> MKPEVEQELAHILLTELLAYQFASPVRWIETQDVFLKDFNTERVVEIGPSPTLAGMAQRTLKNKYESYDAALSLHREILCYSKDAKEIYYTPDPSELAAKEEPAKEEAPAPTPAANAPAPAAAAPAPVAAAAPAAAAAEIADEPVKASLLLHVLVAHKLKKSLDSIPMSKTIKDLVGGKSTVQNEILGDLGKEFGTTPEKPEETPLEELAETFQDTFSGALGKQSSSLLSRLISSKMPGGFTITVARKYLQTRWGLPSGRQDGVLLVALSNEPAARLGSEADAKAFLDSMAQKYASIVGVDLSSAASASGAAGAGAAAGAAMIDAGALEEITKDHKVLARQQLQVLARYLKMDLDNGERKFLKEKDTVAELQAQLDYLNAELGEFFVNGVATSFSRKKARTFDSSWNWAKQSLLSLYFEIIHGVLKNVDREVVSEAINIMNRSNDALIKFMEYHISNTDETKGENYQLVKTLGEQLIENCKQVLDVDPVYKDVAKPTGPKTAIDKNGNITYSEEPREKVRKLSQYVQEMALGGPITKESQPTIEEDLTRVYKAISAQADKQDISSSTRVEFEKLYSDLMKFLESSKEIDPSQTTQLAGMDVEDALDKDSTKEVASLPNKSTISKTVSSTIPRETIPFLHLRKKTPAGDWKYDRQLSSLFLDGLEKAAFNGVTFKDKYVLITGAGKGSIGAEVLQGLLQGGAKVVVTTSRFSKQVTDYYQSIYAKYGAKGSTLIVVPFNQGSKQDVEALIEFIYDTEKNGGLGWDLDAIIPFAAIPEQGIELEHIDSKSEFAHRIMLTNILRMMGCVKKQKSARGIETRPAQVILPMSPNHGTFGGDGMYSESKLSLETLFNRWHSESWANQLTVCGAIIGWTRGTGLMSANNIIAEGIEKMGVRTFSQKEMAFNLLGLLTPEVVELCQKSPVMADLNGGLQFVPELKEFTAKLRKELVETSEVRKAVSIETALEHKVVNGNSADAAYAQVEIQPRANIQLDFPELKPYKQVKQIAPAELEGLLDLERVIVVTGFAEVGPWGSARTRWEMEAFGEFSLEGCVEMAWIMGFISYHNGNLKGRPYTGWVDSKTKEPVDDKDVKAKYETSILEHSGIRLIEPELFNGYNPEKKEMIQEVIVEEDLEPFEASKETAEQFKHQHGDKVDIFEIPETGEYSVKLLKGATLYIPKALRFDRLVAGQIPTGWNAKTYGISDDIISQVDPITLFVLVSVVEAFIASGITDPYEMYKYVHVSEVGNCSGSGMGGVSALRGMFKDRFKDEPVQNDILQESFINTMSAWVNMLLISSSGPIKTPVGACATSVESVDIGVETILSGKARICIVGGYDDFQEEGSFEFGNMKATSNTLEEFEHGRTPAEMSRPATTTRNGFMEAQGAGIQIIMQADLALKMGVPIYGIVAMAATATDKIGRSVPAPGKGILTTAREHHSSVKYASPNLNMKYRKRQLVTREAQIKDWVENELEALKLEAEEIPSEDQNEFLLERTREIHNEAESQLRAAQQQWGNDFYKRDPRIAPLRGALATYGLTIDDLGVASFHGTSTKANDKNESATINEMMKHLGRSEGNPVIGVFQKFLTGHPKGAAGAWMMNGALQILNSGIIPGNRNADNVDKILEQFEYVLYPSKTLKTDGVRAVSITSFGFGQKGGQAIVVHPDYLYGAITEDRYNEYVAKVSAREKSAYKFFHNGMIYNKLFVSKEHAPYTDELEEDVYLDPLARVSKDKKSGSLTFNSKNIQSKDSYINANTIETAKMIENMTKEKVSNGGVGVDVELITSINVENDTFIERNFTPQEIEYCSAQPSVQSSFAGTWSAKEAVFKSLGVKSLGGGAALKDIEIVRVNKNAPAVELHGNAKKAAEEAGVTDVKVSISHDDLQAVAVAVSTKK;> MDAYSTRPLTLSHGSLEHVLLVPTASFFIASQLQEQFNKILPEPTEGFAADDEPTTPAELVGKFLGYVSSLVEPSKVGQFDQVLNLCLTEFENCYLEGNDIHALAAKLLQENDTTLVKTKELIKNYITARIMAKRPFDKKSNSALFRAVGEGNAQLVAIFGGQGNTDDYFEELRDLYQTYHVLVGDLIKFSAETLSELIRTTLDAEKVFTQGLNILEWLENPSNTPDKDYLLSIPISCPLIGVIQLAHYVVTAKLLGFTPGELRSYLKGATGHSQGLVTAVAIAETDSWESFFVSVRKAITVLFFIGVRCYEAYPNTSLPPSILEDSLENNEGVPSPMLSISNLTQEQVQDYVNKTNSHLPAGKQVEISLVNGAKNLVVSGPPQSLYGLNLTLRKAKAPSGLDQSRIPFSERKLKFSNRFLPVASPFHSHLLVPASDLINKDLVKNNVSFNAKDIQIPVYDTFDGSDLRVLSGSISERIVDCIIRLPVKWETTTQFKATHILDFGPGGASGLGVLTHRNKDGTGVRVIVAGTLDINPDDDYGFKQEIFDVTSNGLKKNPNWLEEYHPKLIKNKSGKIFVETKFSKLIGRPPLLVPGMTPCTVSPDFVAATTNAGYTIELAGGGYFSAAGMTAAIDSVVSQIEKGSTFGINLIYVNPFMLQWGIPLIKELRSKGYPIQFLTIGAGVPSLEVASEYIETLGLKYLGLKPGSIDAISQVINIAKAHPNFPIALQWTGGRGGGHHSFEDAHTPMLQMYSKIRRHPNIMLIFGSGFGSADDTYPYLTGEWSTKFDYPPMPFDGFLFGSRVMIAKEVKTSPDAKKCIAACTGVPDDKWEQTYKKPTGGIVTVRSEMGEPIHKIATRGVMLWKEFDETIFNLPKNKLVPTLEAKRDYIISRLNADFQKPWFATVNGQARDLATMTYEEVAKRLVELMFIRSTNSWFDVTWRTFTGDFLRRVEERFTKSKTLSLIQSYSLLDKPDEAIEKVFNAYPAAREQFLNAQDIDHFLSMCQNPMQKPVPFVPVLDRRFEIFFKKDSLWQSEHLEAVVDQDVQRTCILHGPVAAQFTKVIDEPIKSIMDGIHDGHIKKLLHQYYGDDESKIPAVEYFGGESPVDVQSQVDSSSVSEDSAVFKATSSTDEESWFKALAGSEINWRHASFLCSFITQDKMFVSNPIRKVFKPSQGMVVEISNGNTSSKTVVTLSEPVQGELKPTVILKLLKENIIQMEMIENRTMDGKPVSLPLLYNFNPDNGFAPISEVMEDRNQRIKEMY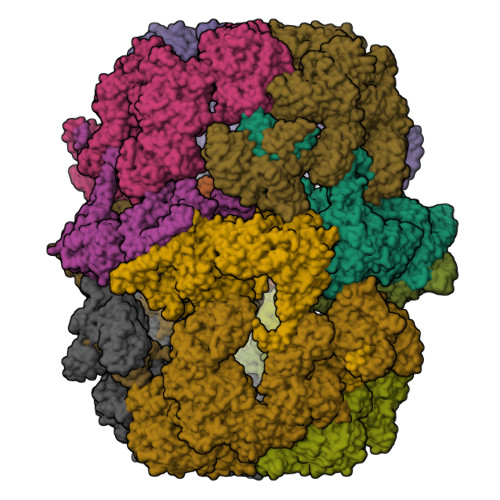WKLWIDEPFNLDFDPRDVIKGKDFEITAKEVYDFTHAVGNNCEDFVSRPDRTMLAPMDFAIVVGWRAIIKAIFPNTVDGDLLKLVHLSNGYKMIPGAKPLQVGDVVSTTAVIESVVNQPTGKIVDVVGTLSRNGKPVMEVTSSFFYRGNYTDFENTFQKTVEPVYQMHIKTSKDIAVLRSKEWFQLDDEDFDLLNKTLTFETETEVTFKNANIFSSVKCFGPIKVELPTKETVEIGIVDYEAGASHGNPVVDFLKRNGSTLEQKVNLENPIPIAVLDSYTPSTNEPYARVSGDLNPIHVSRHFASYANLPGTITHGMFSSASVRALIENWAADSVSSRVRGYTCQFVDMVLPNTALKTSIQHVGMINGRKLIKFETRNEDDVVVLTGEAEIEQPVTTFVFTGQGSQEQGMGMDLYKTSKAAQDVWNRADNHFKDTYGFSILDIVINNPVNLTIHFGGEKGKRIRENYSAMIFETIVDGKLKTEKIFKEINEHSTSYTFRSEKGLLSATQFTQPALTLMEKAAFEDLKSKGLIPADATFAGHSLGEYAALASLADVMSIESLVEVVFYRGMTMQVAVPRDELGRSNYGMIAINPGRVAASFSQEALQYVVERVGKRTGWLVEIVNYNVENQQYVAAGDLRALDTVTNVLNFIKLQKIDIIELQKSLSLEEVEGHLFEIIDEASKKSAVKPRPLKLERGFACIPLVGISVPFHSTYLMNGVKPFKSFLKKNIIKENVKVARLAGKYIPNLTAKPFQVTKEYFQDVYDLTGSEPIKEIIDNWEKYEQSDYKDHDGDYKDHDIDYKDDDDK> MFERFTDRARRVVVLAQEEARMLNHNYIGTEHILLGLIHEGEGVAAKSLESLGISLEGVRSQVEEIIGQGQQAPSGHIPFTPRAKKVLELSLREALQLGHNYIGTEHILL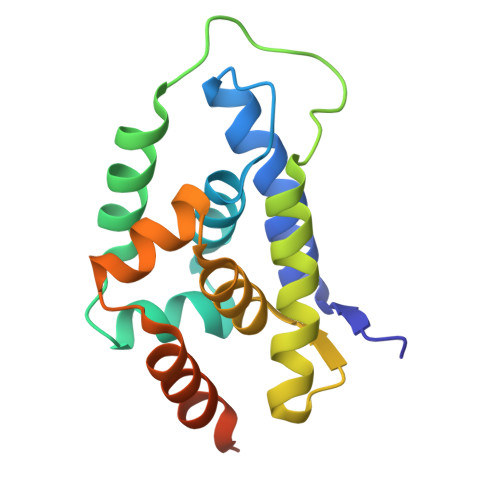GLIREGEGVAAQVLVKLGAELTRVRQQVIQLLSGYKLAAALEHHHHHH> MHHHHHHGENLYFQGSAPYASLTEIEHLVQSVCKSYRETCQLRLEDLLRQRSNIFSREEVTGYQRKSMWEMWERCAHHLTEAIQ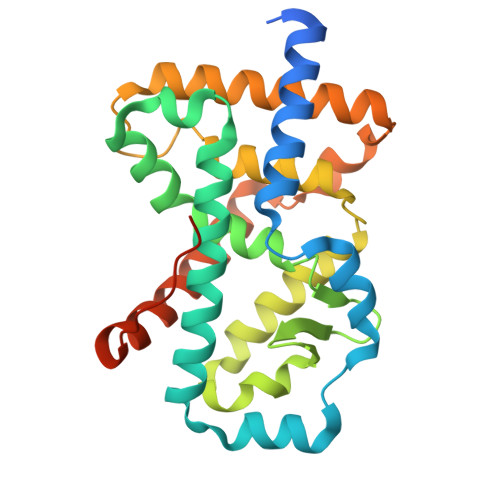YVVEFAKRLSGFMELCQNDQIVLLKAGAMEVVLVRMCRAYNADNRTVFFEGKYGGMELFRALGCSELISSIFDFSHSLSALHFSEDEIALYTALVLINAHRPGLQEKRKVEQLQYNLELAFHHHLCKTHRQSILAKLPPKGKLRSLCSQHVERLQIFQHLHPIVVQAAFPPLYKELFSGNS> SMPKSMQ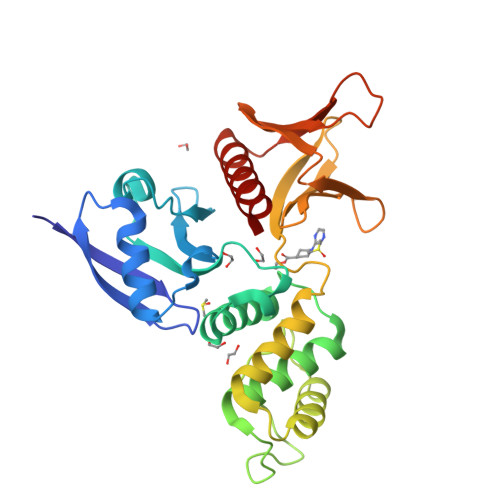CKVILLDGSEYTCDVEKRSRGQVLFDKVCEHLNLLEKDYFGLTYRDAENQKNWLDPAKEIKKQVRSGAWHFSFNVKFYPPDPAQLSEDITRYYLCLQLRDDIVSGRLPCSFVTLALLGSYTVQSELGDYDPDECGSDYISEFRFAPNHTKELEDKVIELHKSHRGMTPAEAEMHFLENAKKLSMYGVDLHHAKDSEGVEIMLGVCASGLLIYRDRLRINRFAWPKVLKISYKRNNFYIKIRPGEFEQFESTIGFKLPNHRAAKRLWKVCVEHHTFFRLL We isolated and characterized two Shigella podophages that have notably different features when compared with classical podophages and instead are most closely related to phage N4. We describe the isolation and characterization of phages Moo19 and B2, including whole-genome sequencing and analysis, cryo–electron microscopy (cryo-EM) structure determination, mass spectrometry, host range studies, and enzymatic assays of the tail proteins. Our work shows that these phages have divergent decoration proteins and unique tail structures, and encode and package their own phage-dependent RNA polymerase, and the tails, which display esterase activity, are dependent on specific O-antigen modifications of lipopolysaccharide (LPS) for entry. Moo19 and B2 are similar to bacteriophage N4—these are all T = 9 podophages, which encapsidate their own polymerases—a hallmark of this phage family.

We also analyzed the data by imposing icosahedral symmetry to visualize the capsids at high resolution (3.6 and 3.4 Å for Moo19 and B2, respectively). Both capsids have a T = 9 geometry (see Fig. 2B for a depiction of the capsid proteins that comprise the asymmetric unit). The major capsid protein of each has the HK97-like fold that is present in most, if not all, dsDNA tailed phages. Using DALI, both the major capsid proteins of Moo19 and B2 are most similar to Ralstonia phage GP4 (37), another T = 9 podophage with an RMSD (root mean square deviation) of 3.0 and 3.2 Å, respectively. The decoration proteins of both Moo19 and B2 bind the capsid proteins at the same quasi-sixfold symmetry axes in both phages but have notably different folds. Moo19’s decoration protein (gp28) displays an immunoglobulin (Ig) domain–like structure that is similar to Hoc in phage T4 (39). The cryo-EM density map of Moo19 was sufficient to clearly model the first 183 amino acids of 273 total residues in gp28. The C-terminal portion is likely also an Ig-like domain that forms the trimer spike similar to Hoc, but the resolution of this region was too poor to accurately model. Whereas the capsids of Moo19, B2, and GP4 are highly similar, it seems that the capsid decoration proteins may stabilize weak points in the capsids in different ways.

>[9x]MLNYNAPIDGQKSSIDGAGSDQMNTFYWLKKAIIQARKDQYFMPLASVTNMPKNMGKTIKVYEYVPLLDDRNINDQGIDANGAHIVNGNLYGSSKDIGTITSKLPLLTENGGRVNRVGFTRLSREGSIHKFGFFYEFTQESLDFDSDDQLKEHLSRELMNGAVQITEAVLQKDLLAAAGTVLYAGAATSDATITGEGSTPSVITYKNLMRLDAILTDNRTPTQTTIITGSRLVDTKVIGGTRVMYVGSELVPDLKAMKDLFGNKAFIEIQHYGDAGTLMNGEIGTIDKFRIIQVPEMLHWAGAGAAATDANPGYRTSTVNGTEHYDVYPVLVVGDDSFTTIGFQTDGKSVKFNVMTKMPGKETADRNDPYGETGFSSIKWYYGILVKRPERIAVMKAVAPL;>[3x]MPELKVAFNKDTYVATVLDASGSVPSGSVNVGTFFHPDETYPDSYVIYHGVRELLYKRSEVDPAQPGFWPENITNMQAVTIDNKATARLVLNTSLPRVVSTIEGGKVTLSVVALGGKAPLKYKWEFRAPNASTWTAVSGQTTANLVLDNIDADKAGEYKVTVTDAAGTSVDSTALVAVGAYPPPALTGIKATPTSLSLSVATDAAGKTVALSAIPTDAELGTLSIKTAPDSARATATISGSTLTVKPVAAGAATSVVVTNGKVDVTITINVAA> AMADLEQKVLEMEASTYDGVFIWKISDFARKRQEAVAGRIPAIFSPAFYTSRYGYKMCLRIYLNGDGTGRGTHLSLFFVVMKGPNDALLRWPFNQKVTLMLLDQNNREHVIDAFRPDVT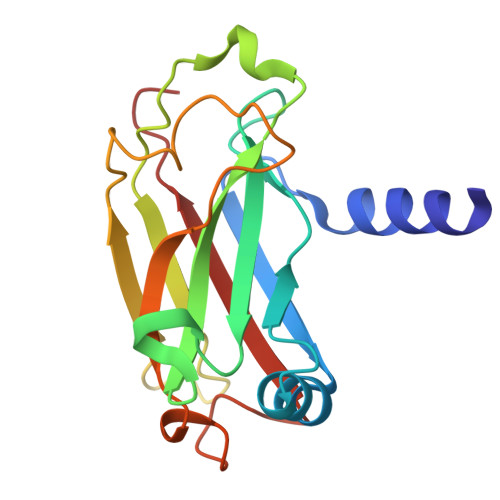SSSFQRPVNDMNIASGCPLFCPVSKMEAKNSYVRDDAIFIKAIVDLTGL> GSMDALNSKEQQEFQKVVEQKQMKDFMRLYSNLVERCFTDCVNDFTTSKLTN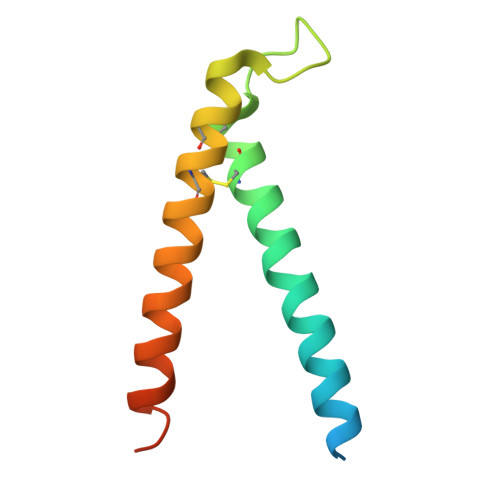KEQTCIMKCSEKFLKHSERVGQRFQEQNAALGQGLGR> GPLHMPGAVGDGPPRVDFPRSRLRFKEKLGEGQFGEVHLCEVDSPQDLVSLDFPLNVRKGHPLLVAVKILRPDATKNARNDFLKEVKIMSRLKDPNIIRLLGVCVQDDPLCMITDYMENGDLNQFLSAHQLEDKAAEGAPGDPTISYPMLLHVAAQIASGMRYLATLNFVHRDLATRNCLVGENFTIKIADFGMSRNLYAGDYYRVQGRAVLPIRWM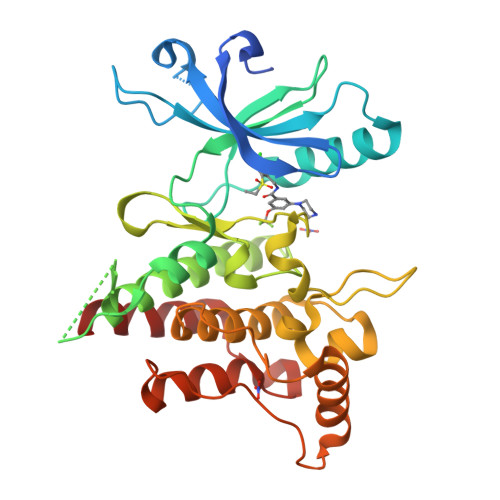AWECILMGKFTTASDVWAFGVTLWEVLMLCRAQPFGQLTDEQVIENAGEFFRDQGRQVYLSRPPACPQGLYELMLRCWSRESEQRPPFSQLHRFLAEDALNTV>GSHMAVQIGFLLFPEVQQLDLTGPHDVLASLPDVQVHLIWKEPGPVVASSGLVLQATTSFADCPPLDVICIPGGTGVGALMEDPQALAFIRQQAARARYVTSVCTGSLVLGAAGLLQGKRATTHWAYHELLAPLGAIPVHERVVRDGNLLTGAGITAGIDFALTLAAELFDAATAQRVQLQLEYAPAPPFNAGSPDTAPASVVQQARQRAADSLHKRREITLRAAARLAAG[2x]

Here, we address each of these questions in a study of diffuse scattering from crystalline isocyanide hydratase (ICH). We selected the ICH system because it diffracts x-rays to atomic resolution at ambient temperature, has clearly visible diffuse features in ambient temperature x-ray diffraction datasets, and displays large concerted motion of an α-helix that is modulated by the chemical state of the active site nucleophile. Upon formation of the catalytic thioimidate intermediate, this helix becomes more mobile and permits water to enter the active site and complete the reaction.

Engineered mutations at residue 150 (e.g., G150A, G150T) also favor shifted conformations of the helix to varying degrees. The refined WT and G150A ICH models are also highly similar (∼0.05–0.07 Å Cα RMSD). In addition, the six WT and G150A datasets show ∼2σ difference (mFo − DFc) electron density features around the mobile helix that indicate a minor population (<10% occupancy) of the shifted helix conformation. The near-identical WT and G150A ICH dimeric protein structures (Cα RMSD ∼ 0.06 Å) provide an opportunity to evaluate the cross correlation coefficient (CCCross) of their diffuse scattering maps. The CCCross for WT-1, for example, can be calculated as the average CC of CC(WT-1, G150A-1), CC(WT-1, G150A-2), and CC(WT-1, G150A-3). We find that the CCCross is ≥0.83 for every WT and G150A dataset, and each data pair within the set of replicate WT and G150A datasets also has CC ≥ 0.8, as shown in orange-colored cells in Table S5. The high cross correlation between WT and G150A diffuse datasets provides additional evidence that protein-derived diffuse scattering is the dominant feature in the processed diffuse anisotropic maps and is consistent with the minor differences in the crystal structures refined against the Bragg data. Despite the Refmac5 and PHENIX models having comparable model statistics and agreement with the Bragg data, the PHENIX models have different distributions of ADP anisotropy. In general, the CCLLM values are higher and σ values are lower for the Refmac5 anisotropic ADP models compared to those refined in PHENIX. By using LLM models that incorporate different anisotropic ADP models for the same structural model, we found that diffuse scattering data can discriminate between more and less plausible representations of anisotropic atomic motion, even when these models have similar Rfree/Rwork and CCBragg values and thus cannot be distinguished easily based on Bragg data alone.>[2x]MNLKDMEQNS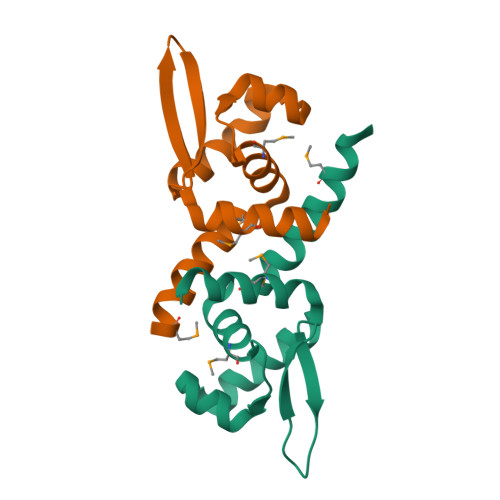AKAVVLLKAMANERRLQILCMLHNQELSVGELCAKLQLSQSALSQHLAWLRRDGLVTTRKEAQTVYYTLKSEEVKAMIKLLHSLYCEE>[4x]GPAMEALELELEEVES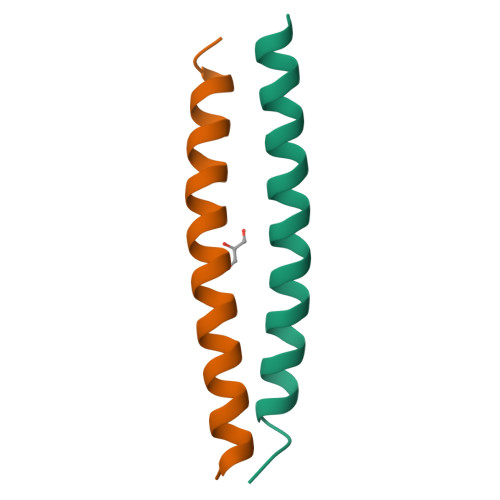QIRALVVRRSRLRERLLAVP>[2x]LLVTPPKALLKPLSIPNQLLLGPGPSNLPPRIMAAGGLQMIGSMSKDMY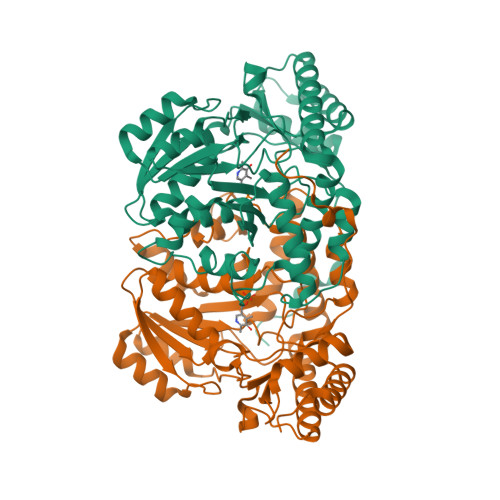QIMDEIKEGIQYVFQTRNPLTLVISGSGHCALEAALVNVLEPGDSFLVGANGIWGQRAVDIGERIGARVHPMTKDPGGHYTLQEVEEGLAQHKPVLLFLTHGESSTGVLQPLDGFGELCHRYKCLLLVDSVASLGGTPLYMDRQGIDILYSGSQKALNAPPGTSLISFSDKAKKKMYSRKTKPFSFYLDIKWLANFWGCDDQPRMYHHTIPVISLYSLRESLALIAEQGLENSWRQHREAAAYLHGRLQALGLQLFVKDPALRLPTVTTVAVPAGYDWRDIVSYVIDHFDIEIMGGLGPSTGKVLRIGLLGCNATRENVDRVTEALRAALQHCPKKK>GSAMGSSSKTSLGLVDLKLFHHYCTEVWPTIIAVGISSPEVWGTYLPDLAFKYPFLMHSMLAFSATHLSRTQPGLDDYVASHRLSALKLLREAVLEISDDNTDALVASSLILIMDSLANASNS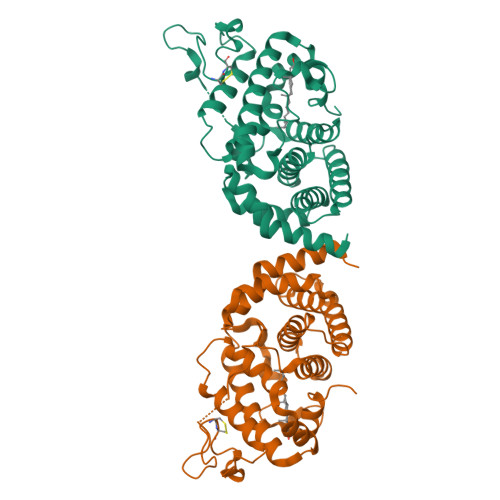NPTAWIFHVKGAVTILTAVWPLPETSKFYNLISVDLSDLGEIVDKDTGTITELVCCDDDIADLYPVDLDSPYLITLAYLDKLYREKNQLDYILRVFAFPALLDRTFLTLLMTGDLGAMRIMRSYYKLLRNYTTEIMDRAWFLEGVSQVLPRDVDDYSGGGGMHMMLDFLGGGLPSMTTTNLSDFM[4x]>MPSSLLGAAMPASTSAAALQEALENAGRLIDRQLQEDRMYPDLSELLMVSAPNNPTVSGMSDMDYPLQGPGLLSVPNLPEISSIRRVPLPPELVEQFGHMQCNCMMGVFPPISRAWLTIDSDIFMWNYEDGGDLAYFDGLSETILAVGLVKPKAGIFQPHVRHLLVLATPVDIVILGLSYANLQTGSGVLNDSLSGGMQLLPDPLYSLPTDNTYLLTITSTDNGRIFLAGKDGCLYEVAYQAEAGWFSQRCRKINHSKSSLSFLVPSLLQFTFSEDDPILQIAIDNSRNILYTRSEKGVIQVYDLGQDGQGMSRVASVSQNAIVSAAGNIARTIDRSVFKPIVQIAVIENSESLDCQLLAVTHAGVRLYFSTCPFRQPLARPNTLTLVHVRLPPGFSASSTVEKPSKVHRALYSKGILLMAASENEDNDILWCVNHDTFPFQKPMMETQMTAGVDGHSWALSAIDELKVDKIITPLNKDHIPITDSPVVVQQHMLPPKKFVLLSAQGSLMFHKLRPVDQLRHLLVSNVGGDGEEIERFFKLHQEDQACATCLILACSTAACDREVSAWATRAFFRYGGEAQMRFPTTLPPPSNVGPILGSPVYSSSPVPSGSPYPNPSFLGTPSHGIQPPAMSTPVCALGNPATQATNMSCVTGPEIVYSGKHNGICIYFSRIMGNIWDASLVVERIFKSGNREITAIESSVPCQLLESVLQELKGLQEFLDRNSQFAGGPLGNPNTTAKVQQRLIGFMRPENGNPQQMQQELQRKFHEAQLSEKISLQAIQQLVRKSYQALALWKLLCEHQFTIIVAELQKELQEQLKITTFKDLVIRDKELTGALIASLINCYIRDNAAVDGISLHLQDICPLLYSTDDAICSKANELLQRSRQVQNKTEKERMLRESLKEYQKISNQVDLSNVCAQYRQVRFYEGVVELSLTAAEKKDPQGLGLHFYKHGEPEEDIVGLQAFQERLNSYKCITDTLQELVNQSKAAPQSPSVPKKPGPPVLSSDPNMLSNEEAGHHFEQMLKLSQRSKDELFSIALYNWLIQVDLADKLLQVASPFLEPHLVRMAKVDQNRVRYMDLLWRYYEKNRSFSNAARVLSRLADMHSTEISLQQRLEYIARAILSAKSSTAISSIAADGEFLHELEEKMEVARIQLQIQETLQRQYSHHSSVQDAVSQLDSELMDITKLYGEFADPFKLAECKLAIIHCAGYSDPILVQTLWQDIIEKELSDSVTLSSSDRMHALSLKIVLLGKIYAGTPRFFPLDFIVQFLEQQVCTLNWDVGFVIQTMNEIGVPLPRLLEVYDQLFKSRDPFWNRMKKPLHLLDCIHVLLIRYVENPSQVLNCERRRFTNLCLDAVCGYLVELQSMSSSVAVQAITGNFKSLQAKLERLH[6x];>MDTEGFGELLQQAEQLAAETEGISELPHVERNLQEIQQAGERLRSRTLTRTSQETADVKASVLLGSRGLDISHISQRLESLSAATTFEPLEPVKDTDIQGFLKNEKDNALLSAIEESRKRTFGMAEEYHRESMLVEWEQVKQRILHTLLASGEDALDFTQESEPSYISDVGPPGRSSLDNIEMAYARQIYIYNEKIVNGHLQPNLVDLCASVAELDDKSISDMWTMVKQMTDVLLTPATDALKNRSSVEVRMEFVRQALAYLEQSYKNYTLVTVFGNLHQAQLGGVPGTYQLVRSFLNIKLPAPLPGLQDGEVEGHPVWALIYYCMRCGDLLAASQVVNRAQHQLGEFKTWFQEYMNSKDRRLSPATENKLRLHYRRALRNNTDPYKRAVYCIIGRCDVTDNQSEVADKTEDYLWLKLNQVCFDDDGTSSPQDRLTLSQFQKQLLEDYGESHFTVNQQPFLYFQVLFLTAQFEAAVAFLFRMERLRCHAVHVALVLFELKLLLKSSGQSAQLLSHEPGDPPCLRRLNFVRLLMLYTRKFESTDPREALQYFYFLRDEKDSQGENMFLRCVSELVIESREFDMILGKLENDGSRKPGVIDKFTSDTKPIINKVASVAENKGLFEEAAKLYDLAKNADKVLELMNKLLSPVVPQISAPQSNKERLKNMALSIAERYRAQGISANKFVDSTFYLLLDLITFFDEYHSGHIDRAFDIIERLKLVPLNQESVEERVAAFRNFSDEIRHNLSEVLLATMNILFTQFKRLKGTSPSSSSRPQRVIEDRDSQLRSQARTLITFAGMIPYRTSGDTNARLVQMEVLMN[4x];>[4x]MATPLAVNSAASLWGPYKDIWHKVGNALWRRQPEAVHLLDKILKKHKPDFISLFKNPPKNVQQHEKVQKASTEGVAIQGQQGTRLLPEQLIKEAFILSDLFDIGELAAVELLLAGEHQQPHFPGLTRGLVAVLLYWDGKRCIANSLKALIQSRRGKTWTLELSPELASMTTRFTDELMEQGLTYKVLTLVSQIDVNNEFEKLQRERGLGSEKHRKEVSDLIKECRQSLAESLFAWACQSPLGKEDTLLLIGHLERVTVEANGSLDAVNLALLMALLYCFDISFIEQSTEERDDMIHQLPLLTEKQYIATIHSRLQDSQLWKLPGLQATVRLAWALALRGISQLPDVTALAEFTEADEAMAELAIADNVFLFLMESVVVSEYFYQEEFYIRRVHNLITDFLALMPMKVKQLRNRADEDARMIHMSMQMGNEPPISLRRDLEHLMLLIGELYKKNPFHLELALEYWCPTEPLQTPTIMGSYLGVAHQRPPQRQVVLSKFVRQMGDLLPPTIYIPYLKMLQGLANGPQCAHYCFSLLKVNGSSHVENIQGAGGSPVSWEHFFHSLMLYHEHLRKDLPSADSVQYRHLPSRGITQKEQDGLIAFLQLTSTIITWSENARLALCEHPQWTPVVVILGLLQCSIPPVLKAELLKTLAAFGKSPEIAASLWQSLEYTQILQTVRIPSQRQAIGIEVELNEIESRCEEYPLTRAFCQLISTLVESSFPSNLGAGLRPPGFDPYLQFLRDSVFLRFRTRAYRRAAEKWEVAEVVLEVFYKLLRDYEPQLEDFVDQFVELQGEEIIAYKPPGFSLMYHLLNESPMLELALSLLEEGVKQLDTYAPFPGKKHLEKAVQHCLALLNLTLQKENLFMDLLRESQLALIVCPLEQLLQGINPRTKKADNVVNIARYLYHGNTNPELAFESAKILCCISCNSNIQIKLVGDFTHDQSISQKLMAGFVECLDCEDAEEFVRLEEGSELEKKLVAIRHETRIHILNLLITSLECNPPNLALYLLGFELKKPVSTTNLQDPGVLGCPRTCLHAILNILEKGTEGRTGPVAVRESPQLAELCYQVIYQLCACSDTSGPTMRYLRTSQDFLFSQLQYLPFSNKEYEISMLNQMSWLMKTASIELRVTSLNRQRSHTQRLLHLLLDDMPVKPYSDGEGGIEDENRSVSGFLHFDTATKVRRKILNILDSIDFSQEIPEPLQLDFFDRAQIEQVIANCEHKNLRGQTVCNVKLLHRVLVAEVNALQGMAAIGQRPLLMEEISTVLQYVVGRNKLLQCLHAKRHALESWRQLVEIILTACPQDLIQAEDRQLIIRDILQDVHDKILDDEAAQELMPVVAGAVFTLTAHLSQAVLTEQKETSVLGPAEAHYAFMLDSCFTSPPPEENPLVGFASIGDSSLYIILKKLLDFILKTGGGFQRVRTHLYGSLLYYLQIAQRPDEPDTLEAAKKTMWERLTAPEDVFSKLQRENIAIIESYGAALMEVVCRDACDGHEIGRMLALALLDRIVSVDKQQQWLLYLSNSGYLKVLVDSLVEDDRTLQSLLTPQPPLLKALYTYESKMAFLTRVAKIQQGALELLRSGVIVRLAQCQVYDMRPETDPQSMFGMRDPPMFIPTPVDRYRQILLPALQLCQVILTSSMAQHLQAAGQVLQFLISHSDTIQAILRCQDVSAGSLQELALLTGIISKAALPGILSELDVDVNEGSLMELQGHIGRFQRQCLGLLSRFGGSDRLRQFKFQDDNVEGDKVSKKDEIELAMQQICANVMEYCQSLMLQSSPTFQHAVCLFTPSLSETVNRDGPRQDTQAPVVPYWRLPGLGIIIYLLKQSANDFFSYYDSHRQSVSKLQNVEQLPPDEIKELCQSVMPAGVDKISTAQKYVLARRRLVKVINNRAKLLSLCSFIIETCLFILWRHLEYYLLHCMPTDSQDSLFASRTLFKSRRLQDSFASETNLDFRSGLAIVSQHDLDQLQADAINAFGESLQKKLLDIEGLYSKVRSRYSFIQALVRRIRGLLRISRN;>[4x]MAFNFGAPSGTSGTAAATAAPAGGFGGFGTTSTTAGSAFSFSAPTNTGTTGLFGGTQNKGFGFGTGFGTTTGTSTGLGTGLGTGLGFGGFNTQQQQQTTLGGLFSQPTQAPTQSNQLINTASALSAPTLLGDERDAILAKWNQLQAFWGTGKGYFNNNIPPVEFTQENPFCRFKAVGYSCMPSNKDEDGLVVLVFNKKETEIRSQQQQLVESLHKVLGGNQTLTVNVEGTKTLPDDQTEVVIYVVERSPNGTSRRVPATTLYAHFEQANIKTQLQQLGVTLSMTRTELSPAQIKQLLQNPPAGVDPIIWEQAKVDNPDSEKLIPVPMVGFKELLRRLKVQDQMTKQHQTRLDIISEDISELQKNQTTSVAKIAQYKRKLMDLSHRTLQVLIKQEIQRKSGYAIQADEEQLRVQLDTIQGELNAPTQFKGRLNELMSQIRMQNHFGAVRSEERYYIDADLLREIKQHLKQQQEGLSHLISIIKDDLEDIKLVEHGLNETIHIRGGVFS;>[4x]MSTGFSFGSGTLGSTTVAAGGTSTGGVFSFGTGASSNPSVGLNFGNLGSTSTPATTSAPSSGFGTGLFGSKPATGFTLGGTNTGIATTITTGLTLGTPATTSAATTGFSLGFNKPAASATPFALPITSTSASGLTLSSALTSTPAASTGFTLNNLGGTTATTTTASTGLSLGGALAGLGGSLFQSTNTGTSGLGQNALGLTLGTTAATSTAGNEGLGGIDFSSSSDKKSDKTGTRPEDSKALKDENLPPVICQDVENLQKFVKEQKQVQEEISRMSSKAMLKVQEDIKALKQLLSLAANGIQRNTLNIDKLKIETAQELKNAEIALRTQKTPPGLQHEYAAPADYFRILVQQFEVQLQQYRQQIEELENHLATQANNSHITPQDLSMAMQKIYQTFVALAAQLQSIHENVKVLKEQYLGYRKMFLGDAVDVFETRRAEAKKWQNTPRVTTGPTPFSTMPNAAAVAMAATLTQQQQPATGPQPSLGVSFGTPFGSGIGTGLQSSGLGSSNLGGFGTSSGFGCSTTGASTFGFGTTNKPSGSLSAGFGSSSTSGFNFSNPGITASAGLTFGVSNPASAGFGTGGQLLQLKKPPAGNKRGKR;>[4x]MSGFNFGGTGAPTGGFTFGTAKTAT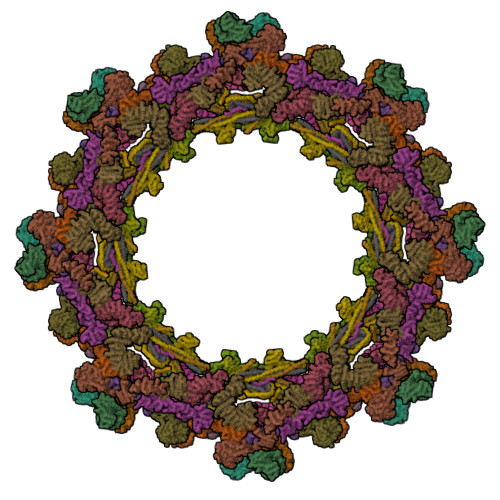TTPATGFSFSTSGTGGFNFGAPFQPATSTPSTGLFSLATQTPATQTTGFTFGTATLASGGTGFSLGIGASKLNLSNTAATPAMANPSGFGLGSSNLTNAISSTVTSSQGTAPTGFVFGPSTTSVAPATTSGGFSFTGGSTAQPSGFNIGSAGNSAQPTAPATLPFTPATPAATTAGATQPAAPTPTATITSTGPSLFASIATAPTSSATTGLSLCTPVTTAGAPTAGTQGFSLKAPGAASGTSTTTSTAATATATTTSSSSTTGFALNLKPLAPAGIPSNTAAAVTAPPGPGAAAGAAASSAMTYAQLESLINKWSLELEDQERHFLQQATQVNAWDRTLIENGEKITSLHREVEKVKLDQKRLDQELDFILSQQKELEDLLSPLEELVKEQSGTIYLQHADEEREKTYKLAENIDAQLKRMAQDLKDIIEHLNTSGAPADTSDPLQQICKILNAHMDSLQWIDQNSALLQRKVEEVTKVCEGRRKEQERSFRITFD> GMQFPSIEDLRARNTMKWTRYGQGVLPLWVAESDFSTCPAVLQAITDAVQREAFGYQPDGSLLSQATAEFYADRYGYQARPEWIFPIPDVVRGLYIAIDHFTPAQSKVIVPTPAYPPFFHLLSATQREGIFIDATGGINLHDVEKGFQAGARSILLCNPYNPLGMVFAPEWLNELCDLAHRYDARVLVDEIHAPLVFDGQHTVAAGVSDTAASVCITITAPSKAWNIAGLKCAQIIFSNPSDAEHWQQL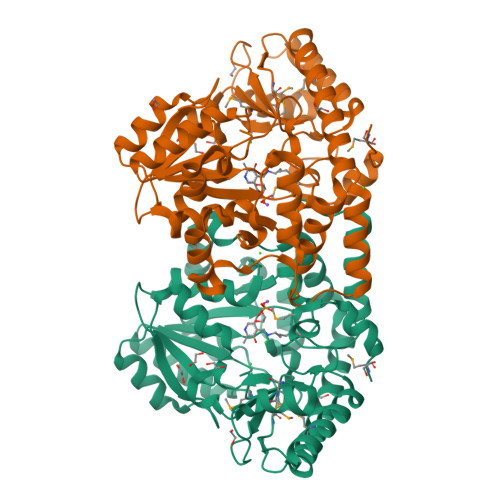SPVIKDGASTLGLIAAEAAYRYGTDFLNQEVAYLKNNHDFLLHEIPKRIPGAKITPMQATYLMWIDFRDTTIEGSPSEFFIEKAKVAMNDGAWFGEDGTGFCRLNFATSREVLEEAIDRMAKAVSHHT> PNGQTKPLPALKLALEYIVPCMN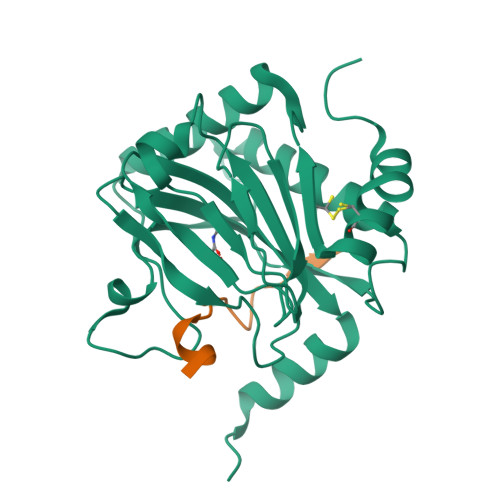KHGICVVDDFLGKETGQQIGDEVRALHDTGKFTDGQLVSQKSDSSKDIRGDKITWIEGKEPGCETIGLLMSSMDDLIRHCNGKLGSYKINGRTKAMVACYPGNGTGYVRHVDNPNGDGRCVTCIYYLNKDWDAKVSGGILRIFPEGKAQFADIEPKFDRLLFFWSDRRNPHEVQPAYATRYAITVWYFDADERAAAKVKYLTGEKGVRVELNKPSDSVGKDVF;> DLEMLAPYIPMDDDFQL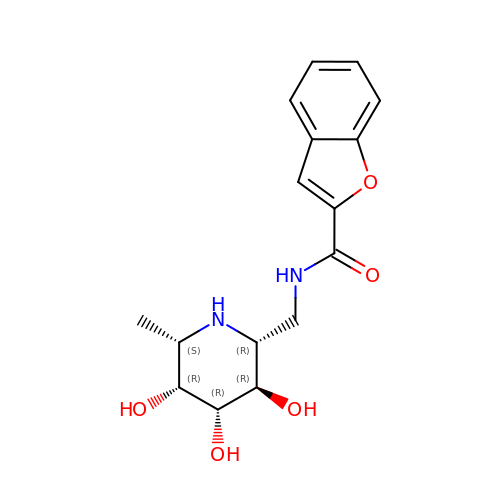N-{[(2R,3R,4R,5R,6S)-3,4,5-trihydroxy-6-methylpiperidin-2-yl]methyl}-1-benzofuran-2-carboxamide | C16 H20 N2 O5 | WSXUKLGXIBOXHU-QFJYNZAASA-N> SNTQAERSIIGMIDMFHKYTRRDDKIDKPSLLTMMKENFPNFLSACDKKGTNYLAGVFEKKDKNEDKKIDFSEFLSLMGDIATDYHKKSHG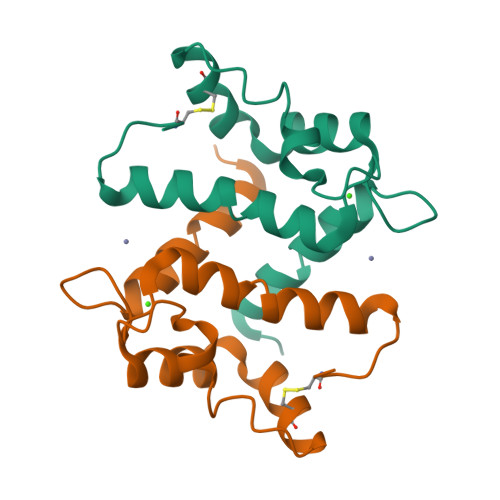AAPCS> MLRQSSLLCFSTFALNPETSRAPHGPPRGLINRYISMGLPPWAAWCNRVNRHALYRMSDVSPRSFLPKAPHEMDVIWMNERVRERVRTSRQVQHVYRQLKYPFVKTGIHYSDTLDHWVQVPMVEAAMFEIEKDGGFDNFIL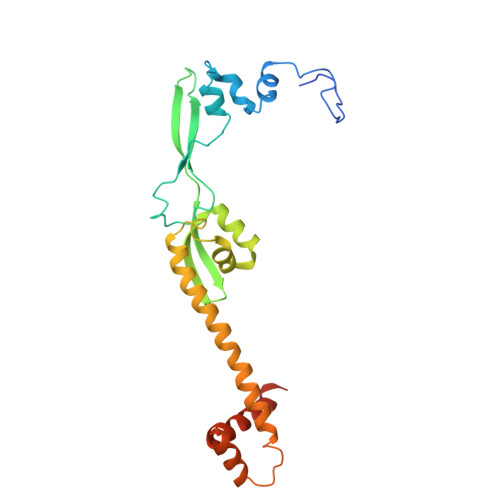KRSGPELRSTYGERIRRHLLVRQKETQKNFVLDQQAKALAEVTQAELMKATSEEELDAVLAKYGMDAEEFKRLMAKRVMEQRKSVAAAGLRSK>[2x]MKLIFLSGVKRSGKDTTADFIMSNYSAVKYQLAGPIKDALAYAWGVFAANTDYPCLTRKEFEGIDYDRETNLNLTKLEVITIM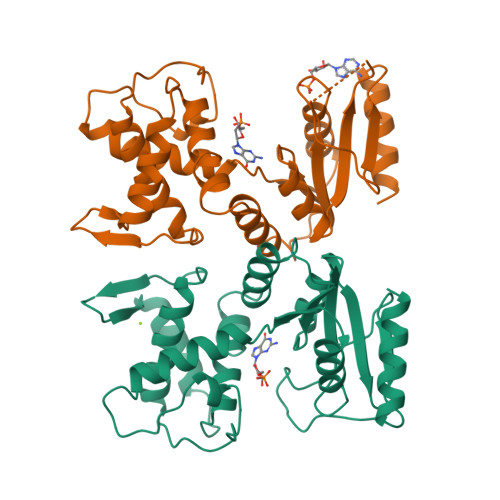EQAFCYLNGKSPIKGVFVFDDEGKESVNFVAFNKITDVINNIEDQWSVRRLMQALGTDLIVNNFDRMYWVKLFALDYLDKFNSGYDYYIVPDTRQDHEMDAARAMGATVIHVVRPGQKSNDTHITEAGLPIRDGDLVITNDGSLEELFSKIKNTLKVL> MITTPLVHVASVEKGRSYEDFQKVYNAIALKLREDDEYDNYIGYGPVLVRLAFHISGTWDKHDNTGGSYGGTYRFKKEFNDPSNAGLQNGFKFLEPIHKEFPWISSGDLFSLGGVTAVQEMQGPKIPWRCGRVDTPEDTTPDNGRLPDADKDAGYVRTFFQRLNMNDREVVALMGAHALGKTHLKNSGYEGPWGAANNVFTNEFYLNLLNEDWKLEKNDANNEQWD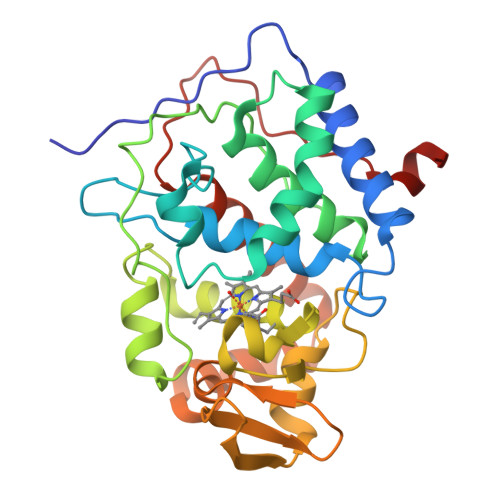SKSGYMMLPTDYSLIQDPKYLSIVKEYANDQDKFFKDFSKAFEKLLENGITFPKDAPSPFIFKTLEEQGL The SNF1 protein kinase complex plays an essential role in regulating gene expression in response to the level of extracellular glucose in budding yeast. SNF1, like AMPK, is a heterotrimeric complex, consisting of a catalytic subunit (Snf1 in yeast; α in mammals) and two regulatory subunits (Sip1, Sip2, or Gal83 in yeast; β in mammals and Snf4 in yeast; γ in mammals) (Hardie, 2007; Hardie et al., 1998). SNF1 activity requires phosphorylation of a threonine residue in the activation loop (T-loop) of the kinase subunit (Thr210), and three protein kinases have been identified that phosphorylate and activate SNF1: Sak1, Elm1, and Tos3 (Hong et al., 2003; Sutherland et al., 2003). Using a tricistronic expression system, we expressed and purified a regulatory fragment of SNF1 from S. cerevisiae comprising the C-terminal domains of Snf1 (457–633) and Sip2 (304–415) together with full-length Snf4 (1–332).

Here we show that ADP is the long-sought metabolite that activates SNF1 in response to glucose limitation by protecting the enzyme against dephosphorylation by Glc7, its physiologically relevant protein phosphatase. We also show that the regulatory subunit of SNF1 has two ADP binding sites. First, we examined nucleotide binding using analogs of ADP and ATP carrying a coumarin fluorescent reporter group in competition assays. These experiments revealed two distinct nucleotide binding sites; AMP, ADP, and ATP bind with similar affinities at a tight site (Kd,I for ADP ∼80 μM) and at a weaker one (Kd,II for ADP ∼800 μM). In order to discover the location of the tight nucleotide binding site on SNF1, we carried out AXP and NADH crystal soaking experiments. Data sets from soaked crystals show strong, well-resolved electron density for AMP, ADP, and NADH at one of the four canonical nucleotide binding sites on Snf4 (labeled site 4 according to the convention suggested by Kemp [Kemp et al., 2007]). The tighter site binds AMP, ADP, and ATP competitively with NADH, whereas the weaker site does not bind NADH, but is responsible for mediating the protective effect of ADP on dephosphorylation. Two lines of evidence lead us to conclude that binding of ADP at the weaker of the two binding sites is responsible for protection of the enzyme against dephosphorylation. Second, the half-maximal effect of ADP on dephosphorylation of SNF1 occurred at a much higher concentration (>500 μM for recombinant SNF1) than the Kd for the tighter binding site (∼80 μM), but close to the Kd of the weaker site. Presumably reflecting the weak binding constant and the lattice packing, we have been unable to obtain crystals of SNF1 with nucleotide present in the weaker site. Given that the linker region is not conserved between mammals and yeast, and that ADP has been shown to bind to site 2 in the S. pombe homolog of AMPK (Jin et al., 2007), we think it is likely that ADP binding at site 2 in Snf4 mediates the protective effect against dephosphorylation of SNF1.

> GPMDQYKEEDSTVSILPTSLPQIHRANMLAQGSPAASKISPLVTKKSKTRWHFGIRSRSYPLDVMGEIYIALKNLGAEWAKPSEEDLWTIKLRWKYDIGNKTNTNEKIPDLMKMVIQLFQIETNNYLVDFKFDGWESSYGDDTTVSNISEDEMSTFSAYPFLHLTTKLIMELAVNSQSN;> MEYTTDIPAVFTDPSVMERYYYTLDRQQSNTDTSWLTPPQLPPQLENVILNKYYATQDQFNENNSGALPIPNHVVLNHLVTSSIKHNTLCVASIVRYKQKYVTQILYTPIESS;> MAKPTQDSQEKVSIEQQLAVESIRKFLNSKTSYDVLPVSYRLIVLDTSLLVKKSLNVLLQNSIVSAPLWDSKTSRFAGLLTTTDFINVIQYYFSNPDKFELVDKLQLDGLKDIERALGVDQLDTASIHPSRPLFEACLKMLESRSGRIPLIDQDEETHREIVVSVLTQYRILKFVALNCRETHFLKIPIGDLNIITQDNMKSCQMTTPVIDVIQMLTQGRVSSVPIIDENGYLINVYEAYDVLGLIKGGIYNDLSLSVGEALMRRSDDFEGVYTCTKNDKLSTIMDNIRKARVHRFFVVDDVGRLVGVLTLSDILKYILLGSN> ASMKETNQKPYKETYGISHITRHDMLQIPEQQKNEKYQVPEFDSSTIKNISSAKGLDVWDSWPLQNADGTVANYHGYHIVFALAGDPKNADDTSIYMFYQKVGETSIDSWKNAGRVFKDSDKFDANDSILKDQTQEWSGSATFTSDGKIRLFYTDFSGKHYGKQTLTTAQVNVSASDSSLNINGVEDYKSIFDGDGKTYQNVQQFIDEGNY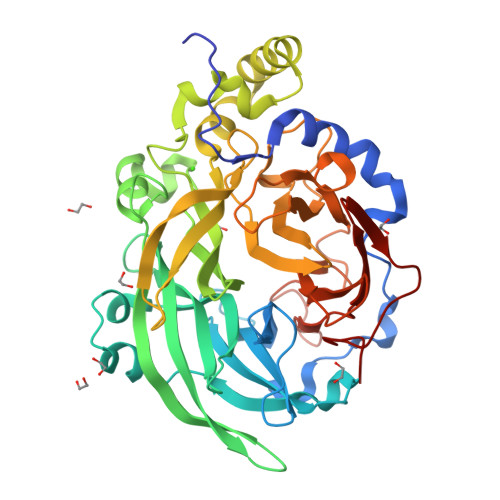SSGDNHTLRDPHYVEDKGHKYLVFEANTGTEDGYQGEESLFNKAYYGKSTSFFRQESQKLLQSDKKRTAELANGALGMIELNDDYTLKKVMKPLIASNTVTDEIERANVFKMNGKWYLFTDSRGSKMTIDGITSNDIYMLGYVSNSLTGPYKPLNKTGLVLKMDLDPNDVTFTYSHFAVPQAKGNNVVITSYMTNRGFYADKQSTFAPSFLLNIKGKKTSVVKDSILEQGQLTVNK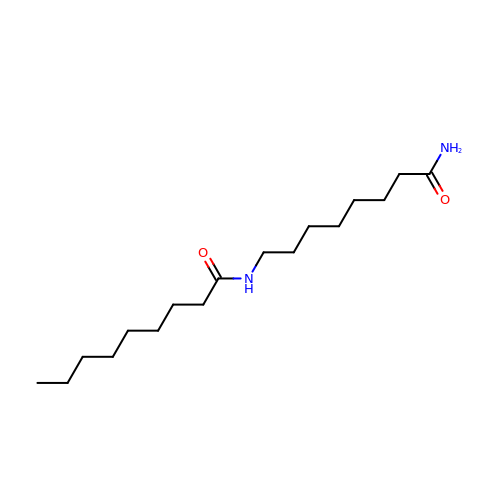N-(8-amino-8-oxooctyl)nonanamide | C17 H34 N2 O2 | SKOHWEXHBDBESR-UHFFFAOYSA-N>MATSLNTIDIQGDILVGMHKQKQLFYFFAINDPATFKTHLASDIAPVVASVTQLSNVATQPLVALNIAFSNTGLLALGVTDNLGDSLFANGQAKDATSFKESTSSWVPQFAGTGIHGVIILASDTTDLIDQQVASIESTFGSSISKLYSLSASIRPGNEAGHEMFGFLDGIAQPAINGFNTPLPGQNIVDAGVIITGATNDPITRPSWAVGGSFLAFRQLEQLVPEFNKYLLDNAPAGSGSLQARADLLGARMVGRWKSGAPIDLTPT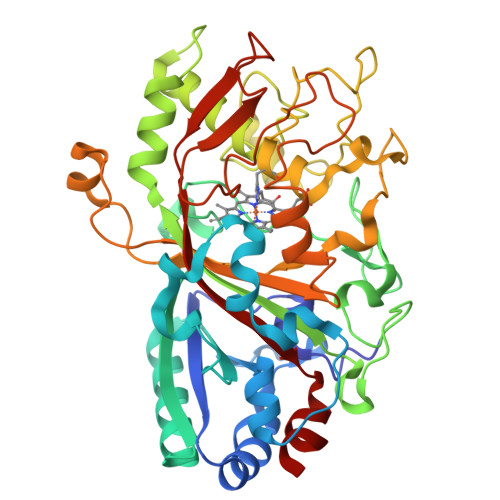ADDPALGADAQRNNNFTYSHAGFDLGSDQSHCPFSAHIRKTRPRADLGGSLTPPNLSAGANSIMRSGIPYGPEVTSAESASNTTTQERGLAFVAYQAQLSQGFHFLQQTWADNANFPPGKTPATVGLDPIIGQNNGQPRVVNGLLPSNSSASLSIPQFVVSHGGEYFFSPPISAIGGRLSA[4x]>EHYSVIQNSLNDKIVTISCKADTNLFFYQVAGNVSLFQQTRNYLERWRLIYDSNKAAYKIKSMDIHNTNLVLTWNAPTHNISTQQDSNADNQYWLLLKDIGNNSFIIASYKNPNLVLYADTVARNLKLSTLNNSNYIKFIIEDYIISDLNNFTCKISPILDLNKVVQQVDVTNLNVNLYTWDYGRNQKWTIRYNEEKAAYQFFNTILSNGVLTWIFSNGNTVRVSSSNDQNNDAQYWLINPVSDTDETYTITNLRDTTKALDLYGGQTANGTAIQVFNYHGDDNQKWNIRNPPGSA[2x];> GPSVERTFLPNGNYNIKSIFSGSLYLNPVSKSLTFSNESSANNQKWNVEYMAENRCFKISNVAEPNKYLSYDNFGFISLDSLSNRCYWFPIKIAVNTYIMLSLNKVNELDYAWDIYDTNENILSQPLLLLPNFDIYNSNQ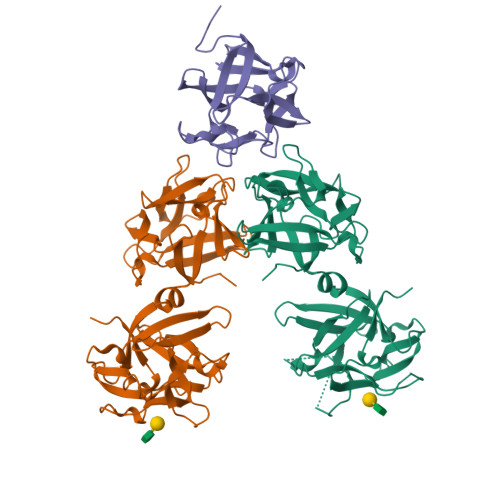MFKLEKI>[2x]MWKDKEFQVLFVLTILTLISGTIFY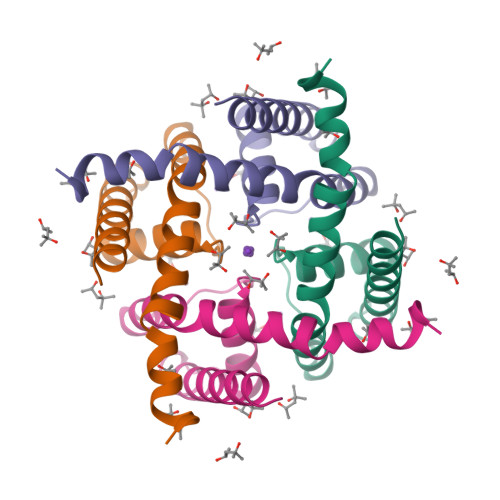STVEGLRPIDALYFSVVTLTTVGCDISPQTDFGKIFTILYIFIGIGLVAGFIHKLAVNVQLPSILSNLVPR> KEKQERVQHLYDIKDLHRYYSSESFEFSNISGKVENYNGSNVVRFNQEKQNHQLFLLGEDKAKYKQGLQGQDVFVVKELIDPNGRLSTVGGVTKKNNQSSETNIHLLVNKLDGGNLDATNDSFLINKEEVSLKEL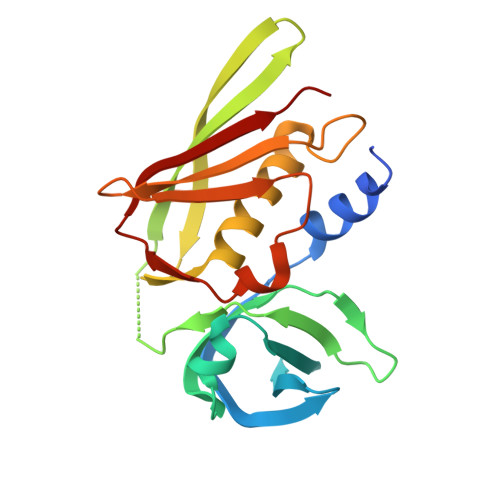DFKIRKQLVEKYGLYQGTSKYGKITIILNGGKKQEIDLGDKLQFERMGDVLNSKDINKIEVTLKQI Pif1 is a DNA helicase belonging to family SF1B of Superfamily 1 (SF1), which unwinds dsDNA with 5′ to 3′ directionality. Pif1 is involved in DNA repair and is necessary for the maintenance of mitochondrial and nuclear genomes integrity, in the regulation of telomerase activity and in the replication fork progression. We were able to crystallize the helicase core of Pif1 from the thermophilic bacteria Deferribacter desulfuricans and Sulfurihydrogenibium sp., which are moderate thermophilic bacteria, living at an average temperature of 65 °C. Pif1 from these bacteria are named DdPif1 and SsPif1, respectively. The helicase core of Pif1 from thermophilic bacteria is very similar to other bacterial Pif1 structures already solved. The HC contains the features of previously described SF1B helicases: two RecA-like domains 1A and 2A containing insertions 1B and 2B, respectively.

By testing different subgroups, it was found that indexing in spacegroup P21 with unit cell a = 113.138 Å b = 129.29Å c = 113.68 Å α = 90 °C β = 103.4 °C γ = 90 °C gave an acceptable MR solution. This spacegroup harbors a strong translational non-crystallographic symmetry (tNCS) and twinning with twin law l, -k, h. An unambiguous solution was found in MR with four molecules in the asymmetric unit. The four molecules are arranged in two dimers related by tNCS. In the dimer, the molecules are related by a non-crystallographic two-fold symmetry, interacting by a β-strand in the 2B domain. The nucleotide binding pocket sits between domains 1A and 2A but most of the interactions with the base involve only domain 1A and the N-terminal tail. The same feature is observed in the SsPif1-ADP structure where the N-terminal part (residues 1-22) participates in ADP binding. The adenine base is stacked by an aromatic residue of motif IV (Y183, Y186 or F187 in DdPif1, SsPif1, and BsPif1, respectively) and a hydrophobic site chain of a residue of the N-terminal tail (A4, V5 or M4 in DdPif1, SsPif1, and BsPif1, respectively). Most of these residues are interacting through their peptidic bond, K28 to 735 for DdPif1 and A31 to T37 for SsPif1. Since the resolution of these structures is limited to 3.2 Å, details of interaction, in particular Mg2+ and water molecules, could not be built.

>[4x]MIQTVEFNEQFSKALDLMENTNKNVLIVGRAGTGKSTLLNYFRNNTKKKIAVLAPTGVAAVNIKGQTIHSFFNFKPDITLSSVKDIKPKNKEIYKKLDAIVIDEVSMVRADLFDCINEFLKIHGKQPGEPFGGIQLILIGDLYQLPPVVTSSEKKFFSQIYKSPFFFDSISFNEAEFEFVELEKVYRQKDEKFIKLLNAIRNKTIEEKDLEELNKRYIPDFEPDEKEFYIYLTTTNELADKINQQKLEKLKGKKYVYQGYIEGDFSEKDLPAPLELVIKKGTQVMLLNNDYQGRWINGSMGRVVDIEKVKGNEDIIWVELEDGEEVPVQPYEWDMFEFYYDKAQKKIKSRTVGSYYQYPLKPAWAITIHKSQGLTFDKVIIDIGRGTFSHGQLYVALSRCRSLEGLVLKKPISEKYIWLDKRVVSFLTKYQYKLSSKKLPLEEKIEIIKKAISEKKPIEIVYLKSKDVKSKRVIIPKKIGKMDYNGAEFLGVEGFCTIRKDDRVFNVEKILEIKEIE> NTGLLESQLSRHDQMLSVHDIRLADMDLRFQVLETASYNGVLIWKIRDYKRRKQEAVMGKTLSLYSQPFYTGYFGYKMCARVYLNGDGMGKGTHLSLFFVIMRGEYDALLPWPFKQKVTLMLMDQGSSRRHLGDAFKPDPNSSSFKKPTGEMNIASGCPVFVAQTVLENGTYIKDDTIFIKVIV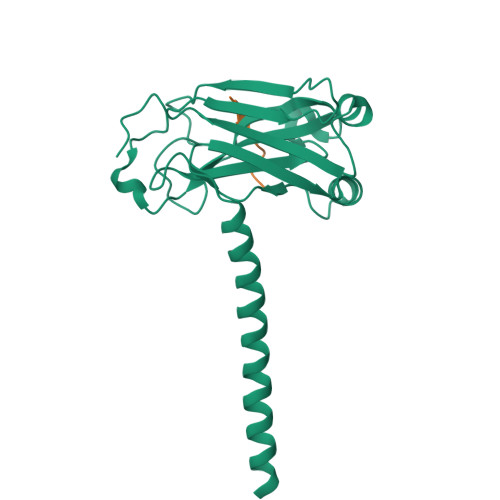DTSDLPDP;> HPQQATDD>MSLDKVMVVAEVRPSEDVNKVLSAISNFFDFEKMNTRKEG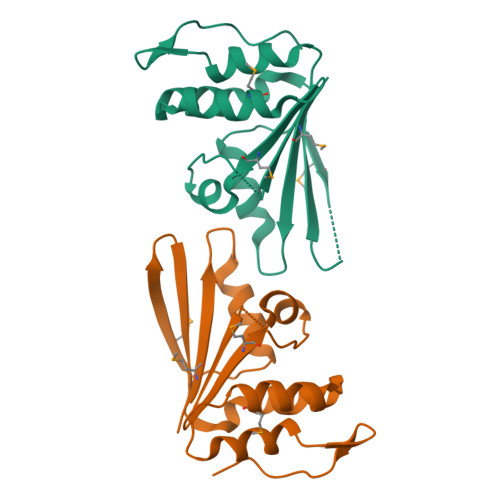IIDILVLEARTLKSLLKFHRVLRNERILDSARKYLMKGIEGNTIAFMIHKQAAAVGVLSFVDSDKESPLGAIKFYIEYQNPKEIVDWLAPKTAHGVPLWDNPVPPDVEGHHHHHH[2x]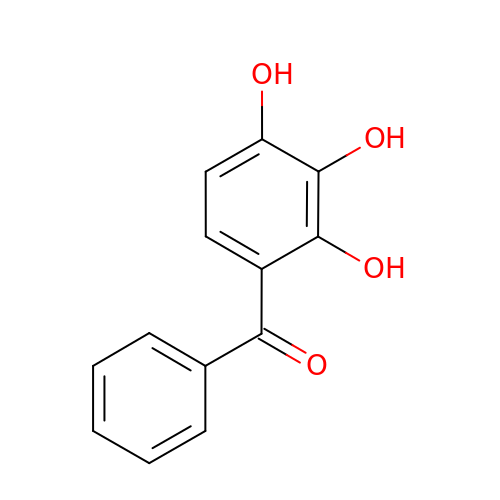2,3,4-Trihydroxybenzophenone | C13 H10 O4 | HTQNYBBTZSBWKL-UHFFFAOYSA-N>MSDKDSKNTPQVPEKLGLSRRGFLGASAVTGAAVAATALGGAVMTRESWAQAVKESKQKIHVGPGELDDYYGFWSGGHQGEVRVLGVPSMRELMRIPVFNVDSATGWGLTNESR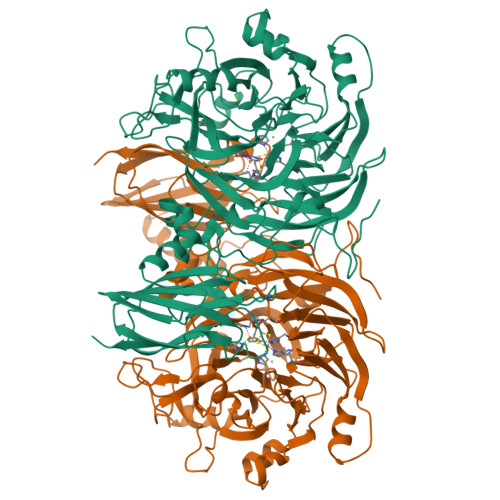HIMGDSAKFLNGDCHHPHISMTDGKYDGKYLFINDKANSRVARIRLDIMKCDKMITVPNVQAIHGLRLQKVPHTKYVFANAEFIIPHPNDGKVFDLQDENSYTMYNAIDAETMEMAFQVIVDGNLDNTDADYTGRFAAATCYNSEKAFDLGGMMRNERDWVVVFDIHAVEAAVKAGDFITLGDSKTPVLDGRKKDGKDSKFTRYVPVPKNPHGCNTSSDGKYFIAAGKLSPTCSMIAIDKLPDLFAGKLADPRDVIVGEPELGLGPLHTTFDGRGNAYTTLFIDSQVVKWNMEEAVRAYKGEKVNYIKQKLDVHYQPGHLHASLCETNEADGKWLVALSKFSKDRFLPVGPLHPENDQLIDISGDEMKLVHDGPTFAEPHDCIMARRDQIKTKKIWDRNDPFFAPTVEMAKKDGINLDTDNKVIRDGNKVRVYMTSMAPAFGVQEFTVKQGDEVTVTITNIDQIEDVSHGFVVVNHGVSMEISPQQTSSITFVADKPGLHWYYCSWFCHALHMEMVGRMMVEPA[8x]> MAASGNVVVTRTTNRVTFETDKASYARAVKQIRQVGKEWEKASDAISKPKKDPAKAYDKSAQQMRLVNKRLAETRAREEKRASERSIALARREAKAKEAIARVSAARIKQQVQQMTSPRAGMSEMKKFYQQQEREAKKANRKATIGMNAASRPMNVTR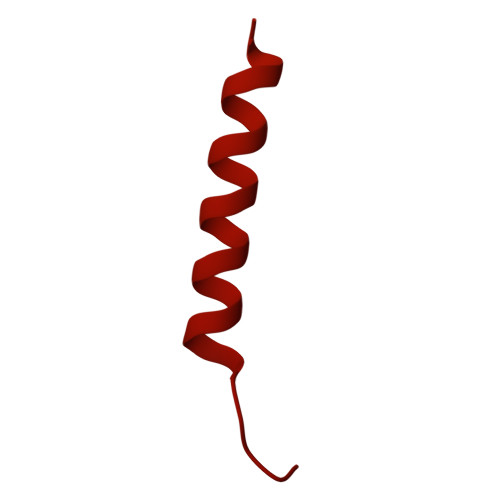INSAPLSPRGGQGTGMVGDPNKVYNPELIAAQNRAMAGRIRSQSQAQDRKAKAEARQRAAAAARAARIDDVMAQQRIRLSSKYGRSYEGRLGRDGAGQGIQDLNRQFRAGTLSAGQYRQSIQALERQFRSAQANAGGFGAALGDIRSQLLNAGAAYGVFASGASVLKQGQFFQGMEATMSMVSDSSEEAGQRIKFVKDQAYRLGLDLKIASQGYTQMAVNSAGILSKAQNDDLFKGFSEFATASQVDPVKFQRGITAIGQMMGKGQVMAEELKGQLAEGIPGSLQVFVKAAQEAFGDTTIDVEKLMDMMQKGELKAAKILPFVGKYFAEAARKGGALPKALESNRVAMQRLSLTWIDFQNQIFQGGFGEQMTRVFRDLATILDSNGELATNLGAFFGNVIEGFWDMVTEIHDDFVLLDRIVSYYTEKLGYQGDLLKEVFDWAGYAIGIGIFVGGLNKIFKILTKIAGLRTALVGVRQAMGGAITRGGVTNGAGLGGGAGAAGTPGASRTASFLSKWKGLSKISKVGILGTLYSAGSMLNEQFIKRGDDKLADAGLDQETFQKEYGFMPKPVGLLDVFDKWFNKPRDLDAPTITAPGPGSGMAAQTGIPFPAPQKVEGDITIKIEAGELRNMVRAVVDENNQFNFNMLIQGGPN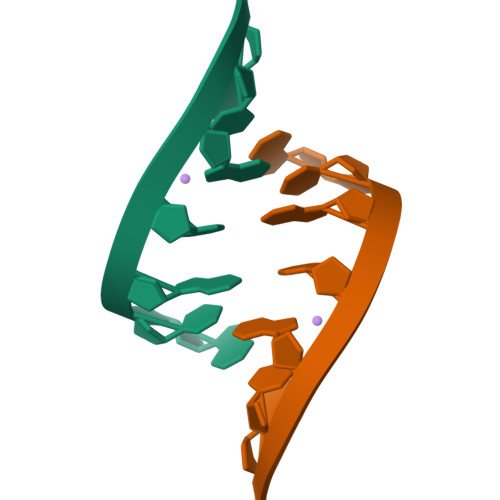>[2x]GUAUACA(3R,5R)-7-[4-(benzylcarbamoyl)-2-(4-fluorophenyl)-5-(1-methylethyl)-1H-imidazol-1-yl]-3,5-dihydroxyheptanoic 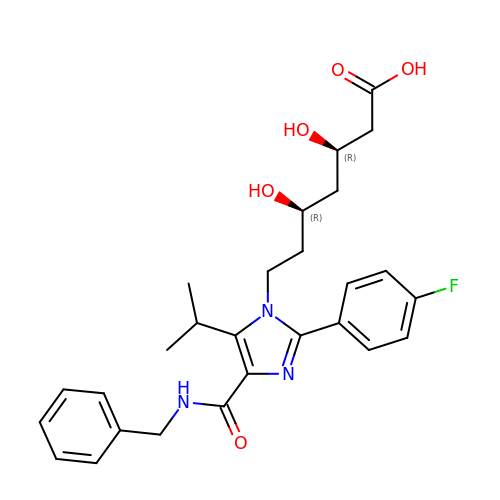acid | C27 H32 F N3 O5 | ATGOOVTXNDYCBK-FGZHOGPDSA-N>MQLFDLPLDQLQTYKPEKTAPKDFSEFWKLSLEELAKVQAEPDLQPVDYPADGVKVYRLTYKSFGNARITGWYAVPDKEGPHPAIVKYHGYNASYDGEIHEMVNWALHGYATFGMLVRGQQRSEDTSISPHGHALGWMTKGILDKDTYYYRGVYLDAVRALEVISSFDEVDETRIGVTGGSQGGGLTIAAAALSDIPKAAVADYPYLSNFERAIDVALEQPYLEINSFFRRNGSPETEVQAMKTLSYFDIMNLADRVKVPVLMSIGLIDKVTPPSTVFAAYNHLET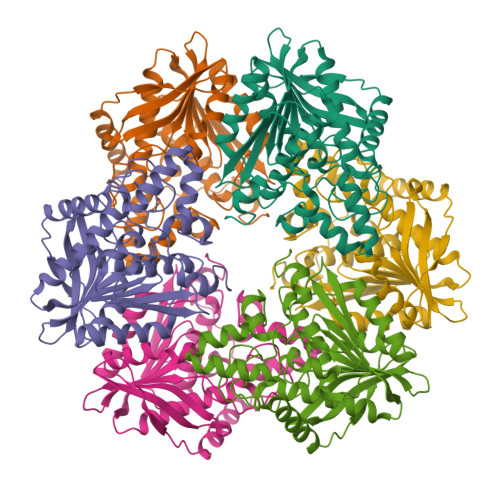KKELKVYRYFGHEYIPAFQTEKLAFFKQILKG[2x]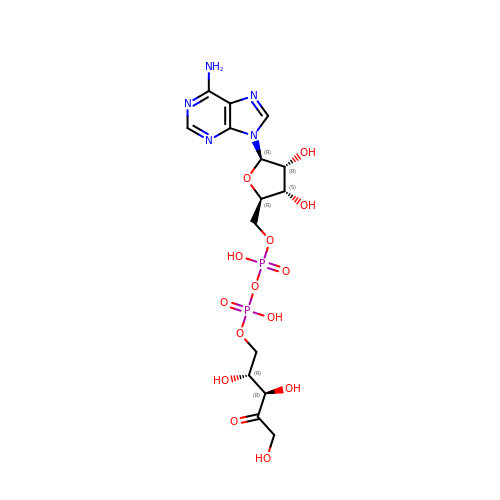[[(2R,3S,4R,5R)-5-(6-aminopurin-9-yl)-3,4-bis(oxidanyl)oxolan-2-yl]methoxy-oxidanyl-phosphoryl] [(2R,3R)-2,3,5-tris(oxidanyl)-4-oxidanylidene-pentyl] hydrogen phosphate | C15 H23 N5 O14 P2 | HMVGRTYSZXZGQZ-GHVQHMAVSA-N>SPIESARIGEVKRETKETNVSVKINLDGHGVSDSSTGIPFLDHMLDQLASHGLFDVHVRATGDTHIDDHHTNEDVALAIGTALLKALGERKGINRFGDFTAPLDEALIHVSLDLSGRPYLGYNLEIPTQRVGTYDTQ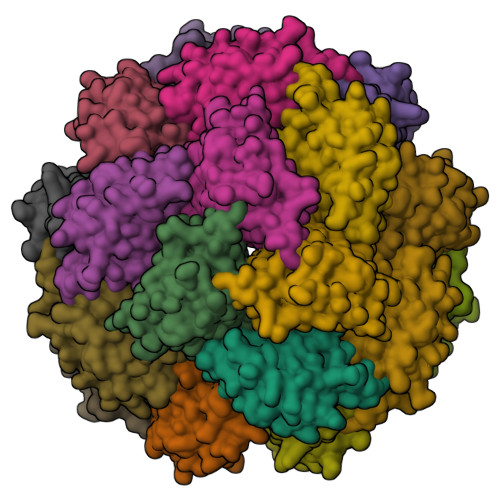LVEHFFQSLVNTSGMTLHIRQLAGKNSHHIIEATFKAFARALRQATESDPRRGGTIPSSKGVLSRS[8x]> MLKQVEIFTDGSCLGNPGPGGYGAILRYKQHEKTFSAGFHLTTNNRMELMAAIVALESLKQPCEVILSTDSQYVRQGITQWIHNWKKRGWKTADKKPVKNVDLW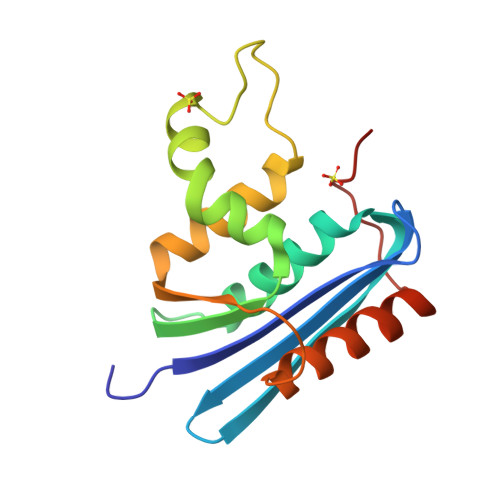QRLDAAIQRHTINWKWVKGHAGHPENERCDELARTAAESPTLEDVGYQPNA Human enteropeptidase (hEP), also known as enterokinase, is an essential enzyme in food digestion and is localized at the brush border of the duodenal and jejunal mucosa. Activated hEP can stimulate the conversion of trypsinogen to trypsin via cleavage of a specific trypsinogen activation peptide, namely Asp-Asp-Asp-Asp-Lys (DDDDK), which is highly conserved in vertebrates. However, the mechanism of hEP activation remains to be established. hEP contains a multi-domain heavy chain and a catalytic light chain, linked by a disulfide bond. The functions of these domains and motifs may be involved in protein anchoring, macromolecular substrate recognition and inhibitor specificity. The light chain is homologous to trypsin-like serine proteinases with a typical Asp-His-Ser (D-H-S) catalytic triad responsible for peptidase activity.

And active hEP incubated with nafamostat was subjected to cryo-EM structure determination. Cryo-EM reconstruction of another ~29% of the particles of the active hEP-nafamostat complex showed an intact hEP with the LCM domain rotated ~120 degrees from the position of the inactive hEP LCM around the loop between MAM and CUB2 domains, with this inhibited hEP LCM in close proximity to the LDLR2 domain. This considerable flexibility was thought to likely facilitate substrate recruitment and expose the catalytic site for subsequent cleavage. The light chain was observed to remain firmly clamped by the CUB2, LDLR2, and SRCR domains of the heavy chain within the core region, allowing for the intimate interaction between the heavy and light chains after the hEP-activating cleavage. The binding of nafamostat or other covalent inhibitors to the catalytic site apparently results in a change of the conformation of the hEP core region. The complex marked by the dashed line displays one of the active states stabilized by the inhibitor.

> ECLPGSSPCTDALTCIKADLFCDGEVNCPDGSDEDNKMCATVCDGRFLLTGSSGSFQATHYPKPSETSVVCQWIIRVNQGLSIKLSFDDFNTYYTDILDIYEGVGSSKILRASIWETNPGTIRIFSNQVTATFLIESDESDYVGFNATYTAFNSSELNNYEKINCNFEDGFCFWVQDLNDDNEWERIQGSTFSPFTGPNFDHTFGNASGFYISTPTGPGGRQERVGLLSLPLDPTLEPACLSFWYHMYGENVHKLSINISNDQNMEKTVFQKEGNYGDNWNYGQVTLNETVKFKVAFNAFKNKILSDIALDDISLTYGICNGSLYPEPTLVPTPPPELPTDCGGPFELWEPNTTFSSTNFPNSYPNLAFCVWILNAQKGKNIQLHFQEFDLENINDVVEIRDGEEADSLLLAVYTGPGPVKDVFSTTNRMTVLLITNDVLARGGFKANFTTGYHLGIPEPCKADHFQCKNGECVPLVNLCDGHLHCEDGSDEADCVRFFNGTTNNNGLVRFRIQSIWHTACAENWTTQISNDVCQLLGLGSGNSSKPIFPTDGGPFVKLNTAPDGHLILTPSQQCLQDSLIRLQCNHKSCGKKLAAQDITPK;> IVGGSNAKEGAWPWVVGLYYGGRLLCGASLVSSDWLVSAAHCVYGRNLEPSKWTAILGLHMKSNLTSPQTVPRLIDEIVINPHYNRRRKDNDIAMMHLEFKVNYTDYIQPICLPEENQVFPPGRNCSIAGWGTVVYQGTTANILQEADVPLLSNERCQQQMPEYNITENMICAGYEEGGIDSCQGDSGGPLMCQENNRWFLAGVTSFGYKCALPNRPGVYARVSRFTEWIQSFLH>PPYTVVYFPVRGRCAALRMLLADQGQSWKEEVVTVETWQEGSLKASCLYGQLPKFQDGDLTLYQSNTILRHLGRTLGLYGKDQQEAALVDMVNDGVEDLRCKYISLIYTNYEAGKDDYVKALPGQLKPFETLLSQNQGGKTFIVADQISFADYNLLDLLLIHEVLAPGCLDAFPLLSAYVGRLSARPKLKAFLASPEYVNLPI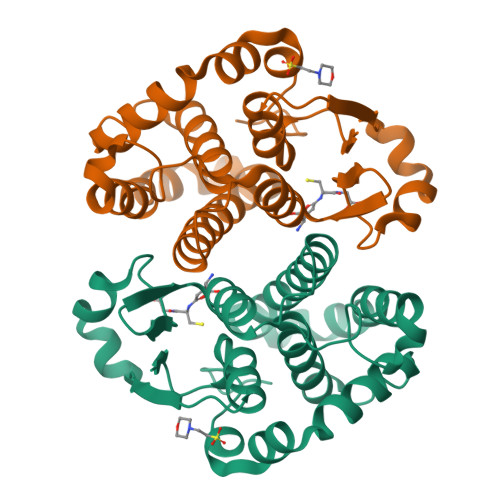NGNGKQ[2x]>MACSAEKQPKPSKQEEEETYSYAMQLASAIVFPAVLQAVIELDVFEIINKAGPGAKLSASEIVAQFPTKNPEAAATMLDRVLRLLVSYNVLYCSLVAGVRLYSLAPVSKYYVRNQNGVSLRPFMNFHLDKALMPCWFRLKEQILEGGSAFHKVHGINFYDYLGTDSRLNEAFNIAMFSQSSIVMDKIIESYKGFDHVNQLVEVGGGLGITLSMIISKYPHIKGINLELPHVIQDAPSYPGVKHVGGDMFERIPEGDTILMKWVFIGFDDDQCLRLLRNCYNAL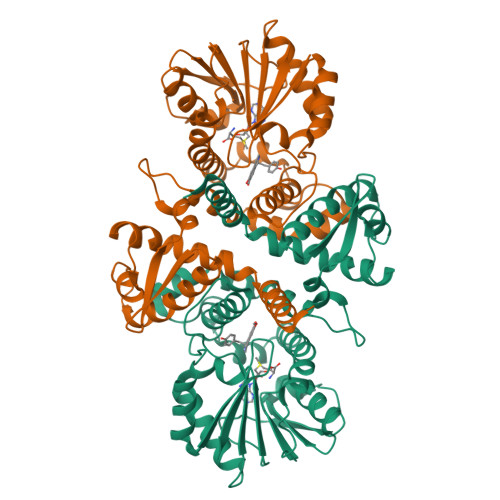PVDGKVLVIDTLLPEVPENSSASRETSNMEAIGLTLVVQGKLRTKQELKALAIEAGFKTINFEYCACNLYVTEFYK[2x]4,5,6,7-TETRACHLORO-PHTHALIDE 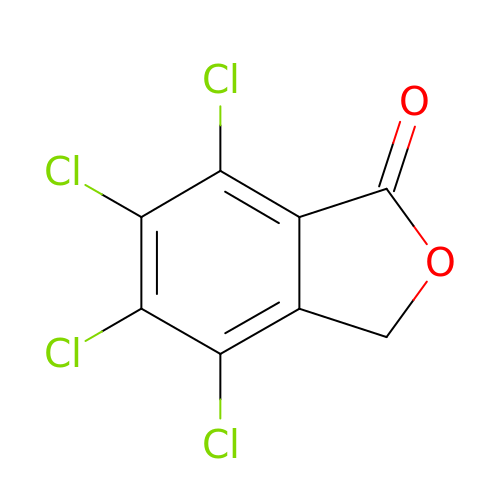| C8 H2 Cl4 O2 | NMWKWBPNKPGATC-UHFFFAOYSA-N> GSGEAE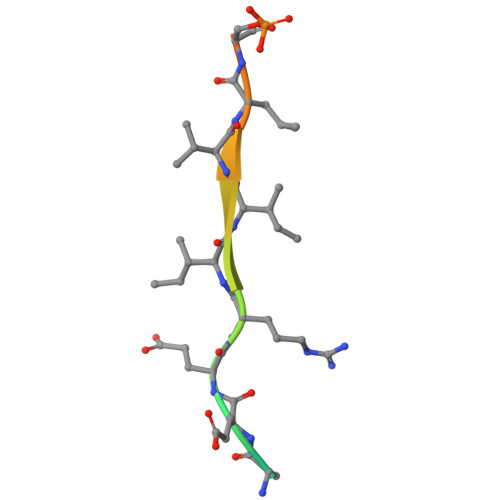ERIIVLSDSDY2-(4,5-dichloro-1H-benzimidazol-2-yl)-5-methyl-4-[(1R)-3-oxo-1,3-dihydro-2-benzofuran-1-yl]-1,2-dihydro-3H-pyrazol-3-one | C19 H12 Cl2 N4 O3 | 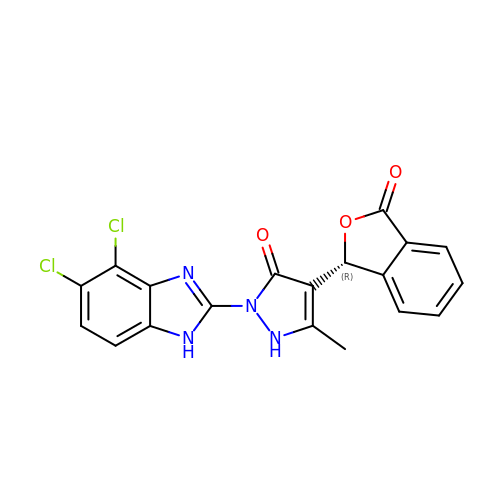IAWZUQAOMURCLV-MRXNPFEDSA-N>[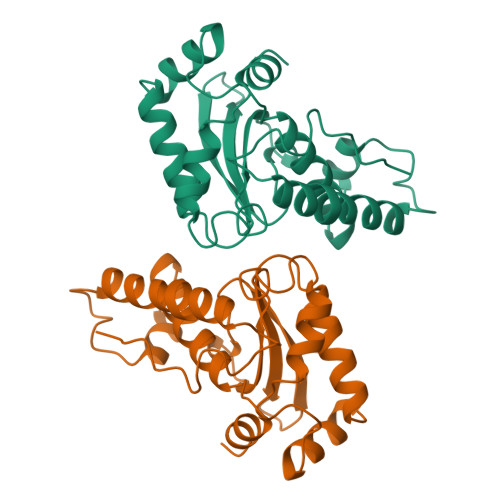2x]SFELPALPYAKDALAPHISAETIEYHYGKHHQTYVTNLNNLIKGTAFEGKSLEEIIRSSEGGVFNNAAQVWNHTFYWNCLAPNAGGEPTGKVAEAIAASFGSFADFKAQFTDAAIKNFGSGWTWLVKNSDGKLAIVSTSNAGTPLTTDATPLLTVDVWEHAYYIDYRNARPGYLEHFWALVNWEFVAKNLAA>[14x]MNLIPTVIETTNRGERA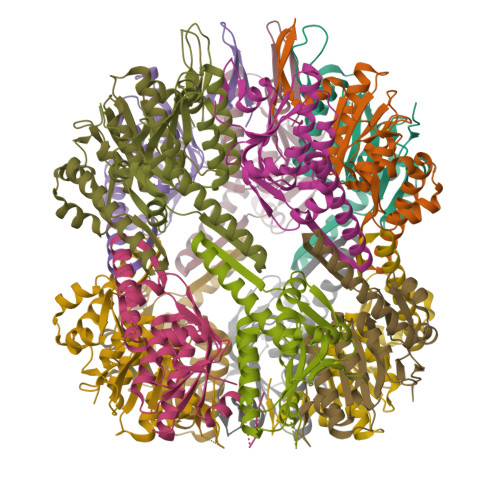YDIYSRLLKDRIIMLGSQIDDNVANSIVSQLLFLQAQDSEKDIYLYINSPGGSVTAGFAIYDTIQHIKPDVQTICIGMAASMGSFLLAAGAKGKRFALPNAEVMIHQPLGGAQGQATEIEIAANHILKTREKLNRILSERTGQSIEKIQKDTDRDNFLTAEEAKEYGLIDEVMVPETK> GNHHHHHMMLIKKIEELKNSEIKDIIDKRIQEFKSFKNKSNEEWFKELCFCILTANFTAEGGIRIQKEIGDGFLTLPREELEEKLKNLGHRFYRKRAEYIVLARRFKNIKDIVESFENEKVAREFLVRNIKGIGYKEASHFLRNVGYDDVAIIDRHI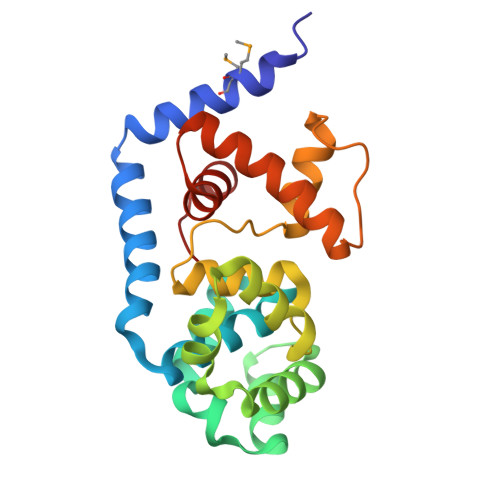LRELYENNYIDEIPKTLSRRKYLEIENILRDIGEEVNLKLSELDLYIWYLRTGKVLK> XAALAAALAQ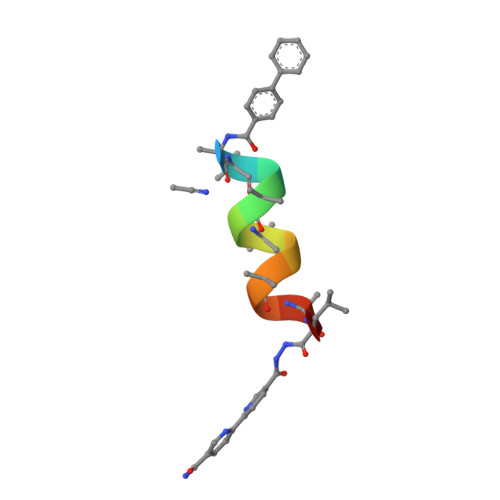ALX>GQEKLYIEKELSWLSFNERVLQEAADKSNPLIERMRFLGIYSNNLDEFYKVRFAELKRRIIISEEQGSNSHSRHLLGKIQSRVLKADQEFDGLYNELLLEMARNQIFLINERQLSVNQQNWLRHYFKQYLRQHITPILINPDTDLVQFLKDDYTYLAVEIIRGDTIRYALLEIPSDKVPRFVNLPPEAPRRRKPMILLDNILRYCLDDIFKGFFDYDALNAYSMKMTRDAEYDLVHEMEASLMELMSSSLKQRLTAEPVRFVYQRDMPNALVEVLREKLTISRYDSIVPGGRYHNFKDFINFPNVGKANLVNKPLPRLRHIWFDKAQFRNGFDAIRERDVLLYYPYHTFEHVLELLRQASFDPSVLAIKINIYRVAKDSRIIDSMIHAAHNGKKVTVVVELQARFDEEANIHWAKRLTEAGVHVIFSAPGLKIHAKLFLISRKENGEVVRYAHIGTGNFNEKTARLYTDYSLLTADARITNEVRRVFNFIENPYRPVTFDYLMVSPQNSRRLLYEMVDREIANAQQGLPSGITLKLNNLVDKGLVDRLYAASSSGVPVNLLVRG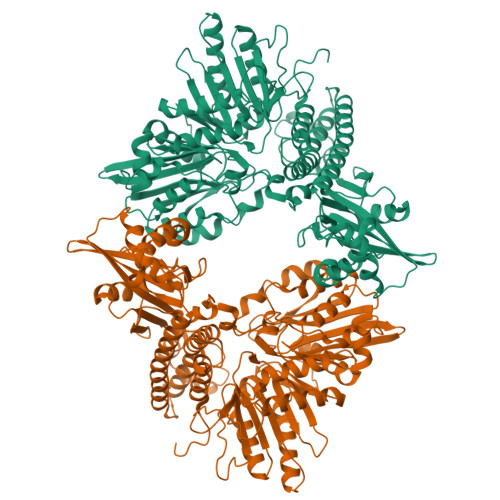MCSLIPNLEGISDNIRAISIVDRYLEHDRVYIFENGGDKKVYLSSADWMTRNIDYRIEVATPLLDPRLKQRVLDIIDILFSDTVKARYIDKELSNRYVPRGNRRKVRAQLAIYDYIKSLEQPE[2x]>GNVARVVVWEWLNEHSRWRPYTATVCHHIENVLKEDARGSVVLGQVDAQLVPYIIDLQSMHQFRQDTGTMRPVRRNFYDPSSAPGKGIVWEWENDGGAWTAYDMDICITIQNAYEKQHPWLDLSSLGFCYLIYFNSMSQMNRQTRRRRRLRRRLDLAYPLTVGSI[2x]

The WWE domain is a relatively under-researched domain found in twelve human proteins and characterized by a conserved tryptophan-tryptophan-glutamate (WWE) sequence motif. Six of these WWE domain-containing proteins also contain domains with E3 ubiquitin ligase activity. Here, we present novel crystal structures of the HUWE1, TRIP12, and DTX1 WWE domains in complex with PAR building blocks and their analogs, thus enabling a comprehensive analysis of the PAR binding site structural diversity. A highly conserved feature in all determined structures is the recognition and therefore the interactions involving the adenine ring of the ligands.

We solved two crystal structures of DTX1 in complex with ADP, with each structure having one ADP molecule bound to either of the two WWE domains. Our efforts to obtain a DTX1 co-crystal structure with both WWE domains bound to ADP were unsuccessful despite having excess ADP in our crystallization setups. To gain insight into why ADP ligands were only observed in one WWE domain in our DTX1-ADP structures, we investigated conformational differences by comparing the bound and unbound WWE domains in the same structure. While the core structural elements appear to be conserved, some loop shifts are observed in both structures, with most differences occurring when ADP is bound to the WWE2 domain as compared to the unbound WWE1 domain in the DTX1-WWE2-ADP structure. The observed differences are in the loops that interact with the phosphate groups and may reduce the surface area of the ligand-binding site in the unbound WWE1 domain of the DTX1-WWE2-ADP structure, which therefore might discourage binding in the second site. This would, however, not be the case in the DTX1-WWE1-ADP structure, as only small conformational differences are observed. Comparing our DTX1-WWE1-ADP and DTX1-WWE2-ADP co-crystal structures with the RNF146-iso-ADPr structure revealed that the residues at the corresponding distal ribose-phosphate moeities binding sites in DTX1 WWE domains may not support high affinity binding to iso-ADPr. Specifically, neither Trp30 nor Trp111 would allow for a direct hydrogen bond to the distal ribose oxygen, while residues in the loop regions (30–38 in WWE1 and 111–122 in WWE2) would not contribute to high affinity binding to the distal phosphate group. Our biophysical data, however, supports DTX1 preference for iso-ADPr over ADPr, which may indicate a mechanism where it recognizes PAR via both iso-ADPr and ADP moieties.>[4x]MGSSHHHHHHSSENLYFQGHMTQRLFVTGLSGFVGKHLQAYLAAAHTPWALLPVPHRYDLLEPDSLGDLWPELPDAVIHLAGQTYVPEAFRDPARTLQINLLGTLNLLQALKARGFSGTFLYISSGDVYGQVAEAALPIHEELIPHPRNPYAVSKLAAESLCLQWGITEGW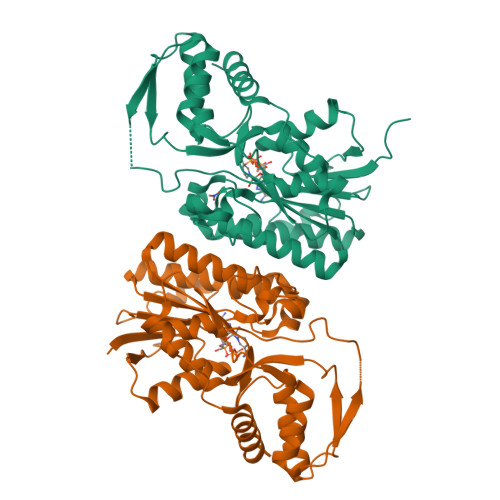RVLVARPFNHIGPGQKDSFVIASAARQIARMKQGLQANRLEVGDIDVSRDFLDVQDVLSAYLRLLSHGEAGAVYNVCSGQEQKIRELIELLADIAQVELEIVQDPARMRRAEQRRVRGSHARLHDATGWKPEITIKQSLRAILSDWESRVREE>MLYEEDYKLALEAFKKVFNALTHYGAKQAFRSRARDLVEEIYNSGFIPTFFYIISKAELNSDSLDSLISLFSSDNAILRGSDENVSYSAYLFIILYYLIKRGIIEQKFLIQALRCEKTRLDLIDKLYNLAPIISAKIRTYLLAIKRLSEALIEAR[3x];>MPYYAFAEPFFIHAITHLHVGSGSSVEEEIDLPFQRDELGYPTIYASSLKGAIKSFLLKEFPDKRDVIYKVLGEDENPEEASLGTFLDAILFAIPSRIIEIDSAKPYVWVYVTTYELLKKVKLYLDSISQLSNASFSNLKNKIDTILAKEGKNITLDSDLKSAILNEDFYVELEALNNKIPSIINAGVPLLVLEDSIGREVINRSLIRVRRIRIDRDKKVVETGGLWSEEYVPMKTIFFSVLLGKESKESAIFASCILRNLRYVILGGKETIGKGIVELRWVKDVI[4x];> MKRVLIKPLEPLMFRSQGEFEPLITGSHTAAQSLIIPRPSTIAGMLGYILFNKSSGTGDWLSDLTNLLATIYGTFIETNGEYLFPLRMGNHLALVDQQHLINLPTLLEKEYERREKGIYELFYDKNKLFQIINHQDRIGISIDKSTRTVKEHYLYSARYLAFKKEVNYVIFIDNDAISDKINGKIVNFGGENRIAKLEVDDYKVDTSIEEEYYLALSPILIPDEALDNFLDNISDYVAMGKVDKISLGFDIANTKRKEMLTAILEGSIVKRSIIDFIKNEIKNDLRYRFSKYEKIGYNTLMSLCKLALRKILS;> MAIDFLVNILELIKEKQCNINLFSAISLTSIVYNNFGEFLSNNQSYSTNNPLLKYHIIILNDKNKTKDVEEKRNIFKREVAELISRNFKLDGEKVRNYFDSLKEVLKSLKYTIVDVEITTRTRALIGVSTSLGKLIFGSGISFDPYMNLPYIPASEIKGIVRSYIEGKLGEQEAEEIFGNEEREGNVNFTDAYPTRSKDFLFVPDVITPHYNGKKSEADAEPRPVIHLTIAPKVTFRFLIYYKREDVGKPICDSMPIILIRGLGARSSVGYSLFELRKIEVIKAAAHHHHHHHHHH;> MEELLMSLKLKALYPLTGGYNRHSINPFYEELVRPTEIKGLWRWWNRVLFNTLAYSTKGKLYTYESIDRLFEDVFGSENKKSAVRLEVITDEGNDNRFELSYVELDKVIDCLRNYKRKVSLDFIDNTLIAEIEGSTKIPISFKSNLDIDKIIKDLVHNNKLLSFELLGFKSVEIDATKISDKKILKEILRDLITNYLEYFNIKQEVTFTLNIYLDKSREHKQNFEDKLKFALYSLLVFILLGGIGRKTSRGFGSLSIIDVKCYDNSICKKIEDLAKNFLKISSGNELKSKIESILDCIKNSCIDTLYIENNILSEIDPKKNVVYFINSDLFEVKRINDKEKVLANIYKAVSSEGCCIKSIITDKYVRKSFLIAFGGYRKVEKDKGLDIGFIKNYLCETCETVSSFNIVDFLLSEGSFMSDYILQYEHRNSLLRFKLISDNSNNSYLIGYILHSSYFKKIDIKYVRCILEKLTYCVI;> MSIDNVLREFLDYKIIALLHDPPNKAWVITGRARNLTQQLSNIRASRKHEKVAKYIINQLFGKNYSEKVDNADKLASSIDRYLGSIVYKERSLFENRSIFLKNILLSNIQRDIGNLFPKDKSKLDNLILEYKKLLNVINKTNLILKYQLFYLIYELVWIDSKYENTPSDTRNPTHTIFDHLYATAAMMNWILSLEKEAKGYLLGIDTIGVADFISKGRKTRDLWISSYLVSALLWYVITWFIEEYGPDVILFPSLRFNQFYAFYLLEKLRKEGVSEDVIDEIKELITKYIFNGDDLFENLKIPPYPIIPGRITLILPGLIREGEEYKKVQDDNCFISKVKERYNEGWRKLIEGLRCYSERKREDGFWNLVCRVLKLTEDLLQTTPLNIRVKQVSVTEDEIFNNNKLRSDSWKIYDNKYRQLVSEFKKSKLVKVTPESRLKLFELTKFDKLPQIGEKSKRGYEFCTSCGVLPAVVIMPKEDELEKKLIDLGIARDEKDVRSIKNMISPGERLCPWCLVKRALGAEPRLMRILLLGDLYSVEKIVNEIVSRDVKIEIPSTSDIASIKTFEEMIEKKNEICEDLKEEEVCEKPSESVLSMWQWFNKNYYNGINLTIDPEEYWFSEKRRRYYFSVFRRHRITFPSPYYALVRADSDYLGDLLEGKLTPYLAGIIDSGDYANISEKKEEVNKLLEEYLVNAGSGSIVDYVKTVLKCIRENLNKCSCAEKIYSNEVAKVMFRVNVEKANVEEEVKNSLEYFETILNEGRIIVTPAWHVSISSALNRGLLVELELVNKHKGFVIYAGGDDLLAMLPVDEVLDFIKESRRAFAGFGTEKLGNMCLENGFVRINNAYYPSLPIVGRSYSVIIAHYADPLFFVINDSYNLLEEGKEIIRYRVMYNGEYKDAKKDVAIFRYQGLTSVIPLSLKRPIVSSVSDFNEIASIIDVILELKKRIDEGRISVSLLYDYEKYKHLIVASDEKYLTEFLVKDWIKRNSLRKHVEFTIDEKLYGVRLTIENYPIKIPNDLISNIVYTLRIIYGGEK;>[26x]MSTQREYVFIPIT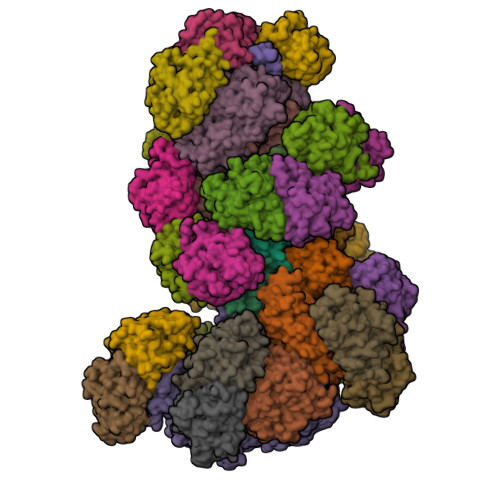NSITIDVKITIGGSDHITNIDERGIHNVLVITGYAVDEKNGRLVPTLDPCDYVKGILVAGTPQQAQSNDFLTLKLPANKLYLIRKKGNISDDLKIYIPYSSPDARNSMKTKPVSISDDTIVNNIIKEVFDKIYNITQKEKVKIEKVKEDIKELFSYYALEQ>HHHHHHHHSQAGDTLNDVIQDPTRRNKLINDNNLLKGIIMGRDGPVPSSRELIVRPDTLRAIINNRATIETTTMEAEFTETLMESNYNSASVKVSAPFITANSEYSESSSFKNTETEKSMYTSSRYLFPQGRIDFTTPDSGFDDVIKLSPQFTSGVQAALAKATGTEKREALQNLFQEYGHVFRTKVHIGGVLSAHTMETFSRSENETEVKQDVKAGLEGAVKGWGGGATAGHGNTQGTITTSQNRKLNVKYIVNGGDYTKIQNTEEWVASTNQSEHWRVIEVTEVTAVADLLPQPIRGQVKDLLKPLLGKWVDVEKVPGLESLPVSVYRPKGAIPAGWFWLGDTADASKALLVKPTLPARSGRNPALTSLHQGSGMTEQPFVDLPQYQYLSTYFGSFAHDTPPGSTLRGLRPDHVLPGRYEMHGDTISTAVYVTRPVDVPFPEDECFDLKSLVRVKLPGSGNPPKPRSALKKSMVLFDSGEK[13x];>[26x]MAYAQWVIIIIHNVGSQDVKIKNLKASWGKLHADGDKDAEVSASNYEGKIVKPDEKLQINASGRSDAAEGTTGTFD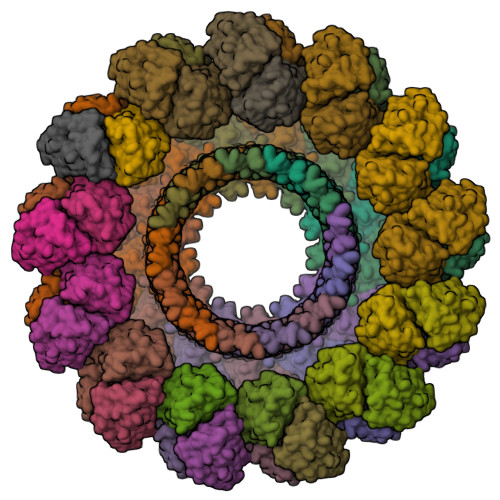LVDPADGDKQVRHFYWDSPWGSKTNTWTVSGSNTKWMIEYSGQNLDSGALGTITVDTLKKGENLYFQ4-METHYL-N-METHYL-N-(2-PHENYL-2H-PYRAZOL-3-YL)BENZENESULFONAMIDE 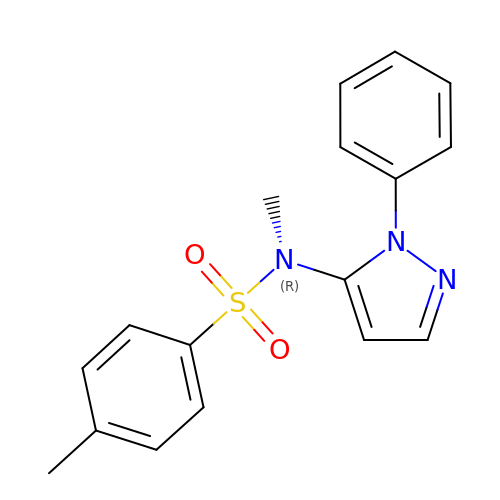| C17 H17 N3 O2 S | KRHPBWNETCEFGS-UHFFFAOYSA-N> DDKMDYDFKVKLSSERERVEDLFEYEGCKVGRGTYGHVYKAKRKDGKDDKDYALKQIEGTGISMSACREIALLRELKHPNVISLQKVFLSHADRKVWLLFDYAEHDLWHIIKFHRASKANKKPVQLPRGMVKSLLYQILDGIHYLHANWVLHRDLKPANILVMGEGPERGRVKIADMGFARLFNSPLKPLADLDPVVVTFWYRAPELLLGARHYTKAIDIWAIGCIFAELLTSEPIFHCRQEDIKTSNPYHHDQLDRIFNVMGFPADKDWEDIKKMPEHSTLMKDFRRNTYTNCSLIKYMEKHKVKPDSKAFHLLQKLLTMDPIKRITSEQAMQDPYFLEDPLPTSDVFAGCQIPYPKREFLTEEEPDDKGDKKNQQQQQGN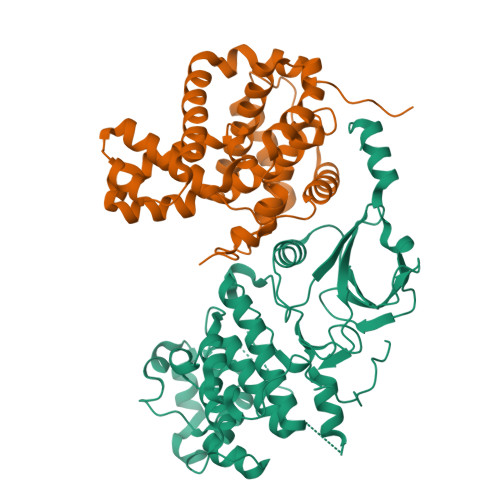NHTNGTGHPGNQDSSHTQGPPLKK;> DKAMAGNFWQSSHYLQWILDKQDLLKERQKDLKFLSEEEYWKLQIFFTNVIQALGEHLKLRQQVIATATVYFKRFYARYSLKSIDPVLMAPTCVFLASKVEEFGVVSNTRLIAAATSVLKTRFSYAFPKEFPYRMNHILECEFYLLELMDCCLIVYHPYRPLLQYVQDMGQEDMLLPLAWRIVNDTYRTDLCLLYPPFMIALACLHVACVVQQKDARQWFAELSVDMEKILEIIRVILKLYEQWKNFDERKEMATILSKMPKPKPPPNSEGEQGPNGSQNSSYSQS>VG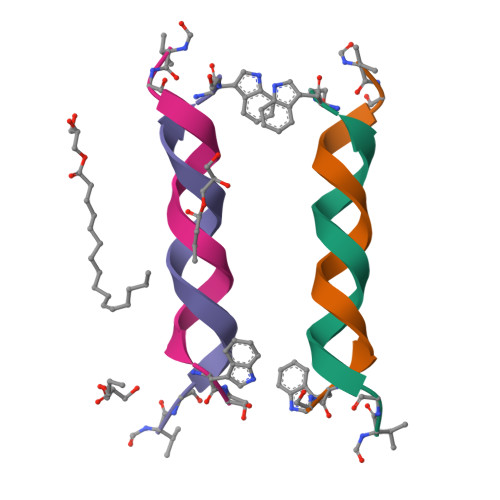ALAVVVWLWLWLWX[4x]> MNINVPDATRIGRATGAKAPEFQELYDFDAAALTLTSAVFPYDSQIHRAHVVMLTEQGILTVEESATILSGLAQVDELAATDGSLRTYLPYEAALKRTIGSVAGKMHIGRSRNDLANAGKRMFLRDQLLRTIEAVIGYREAVVHKAADHLDTVMVVYTQRKEAQPITLGHYLMAISENLAKNLDRYRELYARINLCPLGAAATAGTGWPLNRDRTSALLGFDGLVVNSIEGVAGWDHVAEHAFVNAVFL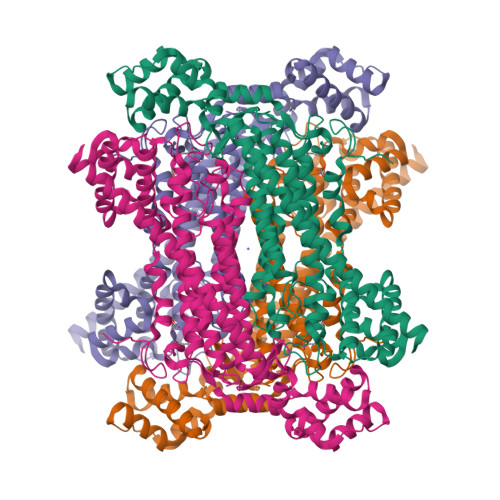SGLSRLASEIQLWSTDEYQVAELDASFAGTSSIMPQKKNPMSLERSRKAAFAAMGPLVGILTSLNAIEYQMSAARVELEPRSIDALIAATHAMTGVVRTLHPNKERMRQYAAENYSTMTDLTDMLVRRVGIDYREAHEIVAHVVITAIEKGIKANKIGLDLVQEAAVAQTGAGINVSADDIKDALDPWQNVLRREGKGMPAPMSVKASIDDAMAELHKDRAWLANATQALANAKQTLADSVQQIIQTDRKYLRHHHHHH>GASHAAILEESMHARDQLMEQNFALDKARQEAEMAVHARNDFLAVMNHEMRTPMHAIISLSSLLLETELSPEQRVMIETILKSSNLVATLISDVLDLSRL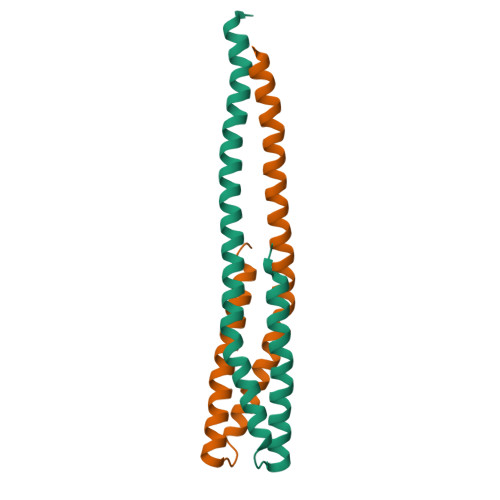ED[2x]N-PROPARGYL-1(S)-AMINOINDAN 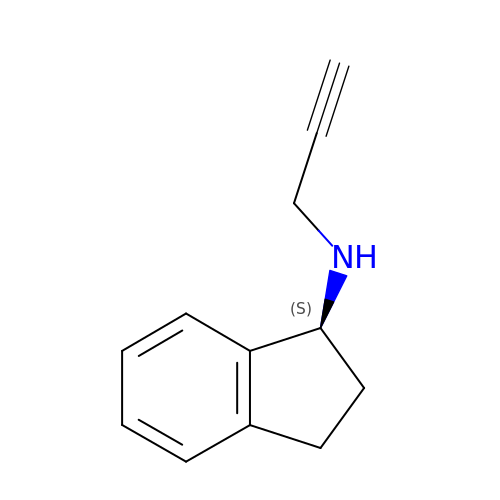| C12 H13 N | RUOKEQAAGRXIBM-LBPRGKRZSA-N> MGHHHHHHGNITLTKRQQEFLLLNGWLQLQCGHAE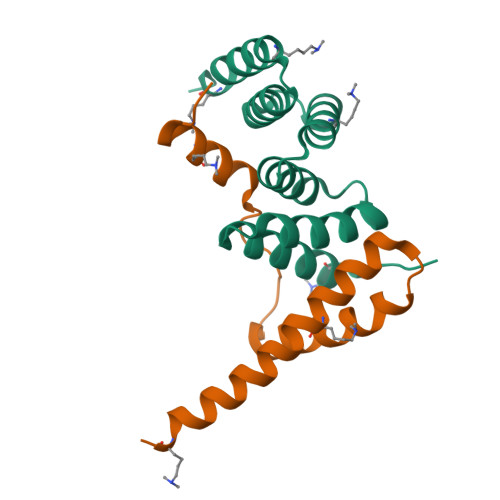RACILLDALLTLNPEHLAGRRCRLVALLNNNQGERAEKEAQWLISHDPLQAGNWLCLSRAQQLNGDLDKARHAYQHYLELKDHNESP;> GAMGALPPDGHPVEPHLERLYPTAQSKRSLWDFASPGYTFHGLHRAQDYRRELDTLQSLLTTSQSSELQAAAALLKCQQDDDRLLQIILNLLHKV> AAPGKPTIAWGNTKFAIVEVDQAATAYNNLVKVKNAADVSVSWNLWNGDTGTTAKVLLNGKEAWSGPSTGSSGTANFKVNKGGRYQMQVALCNADGCTASDATEIVVADTDGSHLAPLKEPLL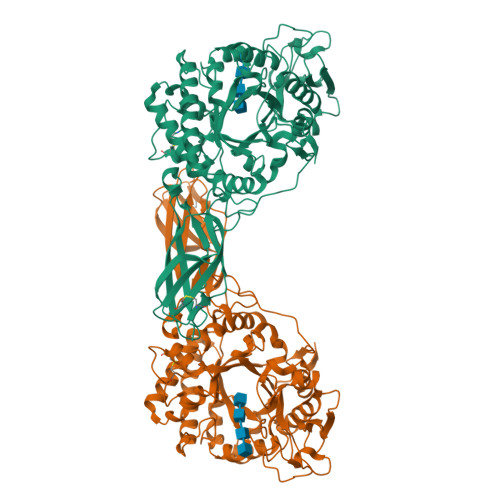EKNKPYKQNSGKVVGSYFVEWGVYGRNFTVDKIPAQNLTHLLYGFIPICGGNGINDSLKEIEGSFQALQRSCQGREDFKVSIHDPFAALQKAQKGVTAWDDPYKGNFGQLMALKQAHPDLKILPSIGGWTLSDPFFFMGDKVKRDRFVGSVKEFLQTWKFFDGVDIDWEFPGGKGANPNLGSPQDGETYVLLMKELRAMLDQLSVETGRKYELTSAISAGKDKIDKVAYNVAQNSMDHIFLMSYAFYGAFDLKNLGHQTALNAPAWKPDTAYTTVNGVNALLAQGVKPGKIVVGTAMYGRGWTGVNGYQNNIPFTGTATGPVKGTWENGIVDYRQIAGQFMSGEWQYTYDATAEAPYVFKPSTGDLITFDDARSVQAKGKYVLDKQLGGLFSWEIDADNGDILNSMNASLGNSAGVQ2-deoxy-6-O-phosphono-beta-D-glucopyranose | C6 H13 O8 P | 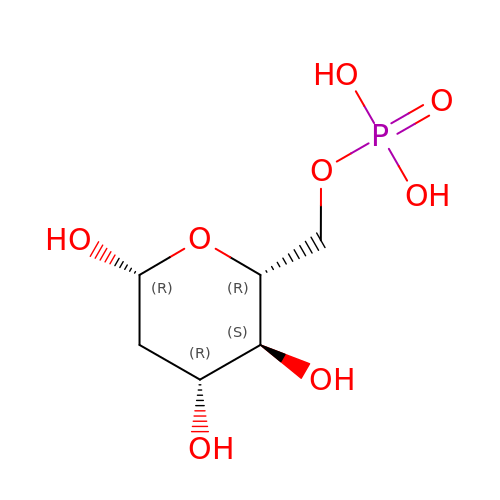UQJFZAAGZAYVKZ-KAZBKCHUSA-N> DT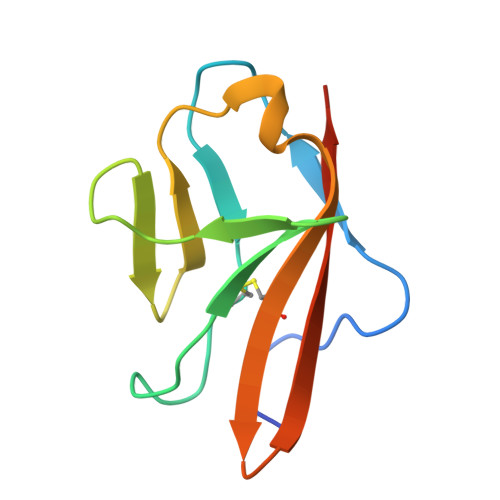GRPFVEMYSEIPEIIHMTEGRELVIPCRVTSPNITVTLKKFPLDTLIPDGKRIIWDSRKGFIISNATYKEIGLLTCEATVNGHLYKTNYLTHRQTNTI> MEKDGLCRADQQYECVAEIGEGAYGKVFKARD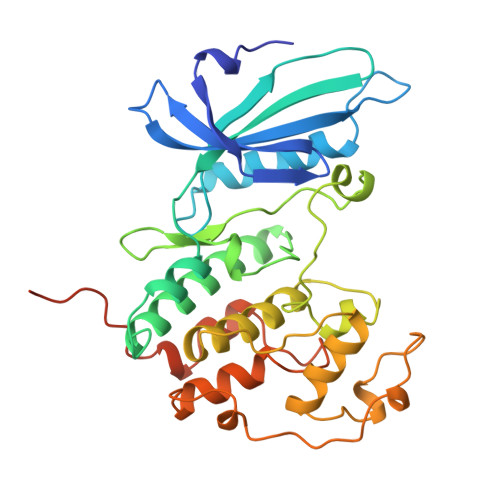LKNGGRFVALKRVRVQTGEEGMPLSTIREVAVLRHLETFEHPNVVRLFDVCTVSRTDRETKLTLVFEHVDQDLTTYLDKVPEPGVPTETIKDMMFQLLRGLDFLHSHRVVHRDLKPQNILVTSSGQIKLADFGLARIYSFQMALTSVVVTLWYRAPEVLLQSSYATPVDLWSVGCIFAEMFRRKPLFRGSSDVDQLGKILDVIGLPGEEDWPRDVALPRQAFHSKSAQPIEKFVTDIDELGKDLLLKCLTFNPAKRISAYSALSHPYFQDLERCKENLDSHLPPSQNTSELNTA>[2x]GSHMTARTPDAEPPLLTPAEVATMFRVDPKTVT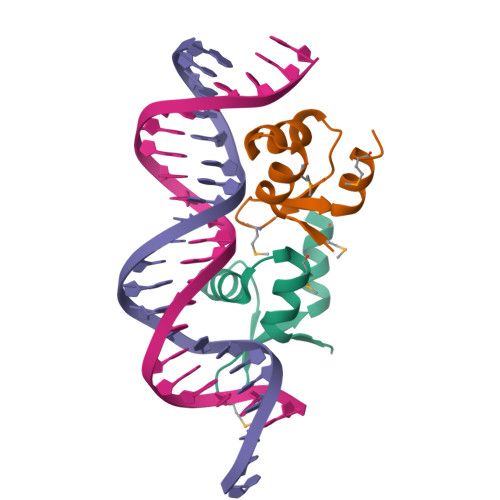RWAKAGKLTSIRTMGGHRRYREAEVRALMAGIPQQRSEA> MGNIRVYCRIRPALKNLENSDTSLIN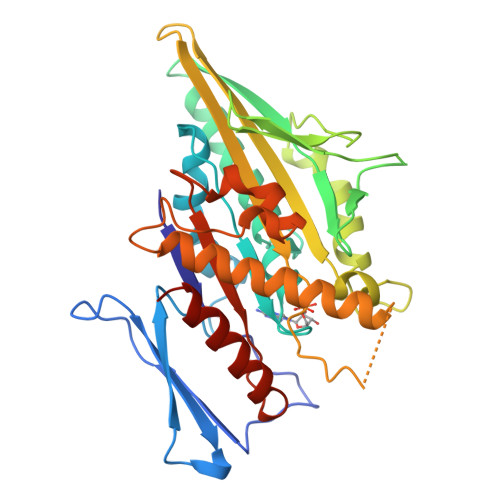VNEFDDNSGVQSMEVTKIQNTAQVHEFKFDKIFDQQDTNVDVFKEVGQLVQSSLDGYNVCIFAYGQTGSGKTFTMLNPGDGIIPSTISHIFNWINKLKTKGWDYKVNCEFIEIYNENIVDLLRSDNNNKEDTSIGLKHEIRHDQETKTTTITNVTSCKLESEEMVEIILKKANKLRSTASTASNEHSSRSHSIFIIHLSGSNAKTGAHSYGTLNLVDLAGSERINVSQVVGDRLRETQNINKSLSCLGDVIHALGQPDSTKRHIPFRNSKLTYLLQYSLTGDSKTLMFVNISPSSSHINETLNSLRFASKVNSTRLVSRK Angiogenin (ANG), a 14-kDa basic protein is an angiogenic ribonuclease and member of the bovine pancreatic ribonuclease (RNase A) family (also known as RNase 5). Like RNase A, ANG cleaves preferentially on the 3′ side of pyrimidines and follows a transphosphorylation/hydrolysis mechanism. In addition, the crystal structure of human ANG has revealed that it has an RNase A fold and the catalytic triad (residues H13, K40 and H114) is conserved. The enzymatic activity of ANG is several orders of magnitude lower than that of RNase A towards conventional RNase substrates, but essential for its angiogenic effect.

ANG residues H13, K40 and H114 (part of the P1 sub-site) correspond to the catalytic triad. In the crystal structure of H13R ANG PD variant, the substitution of H13 by Arg is very clear in the electron density map and the overall structure is largely the same as with native ANG. In the native structure, Nδ1 of H13 forms a hydrogen bond with the main-chain O of T44 and Nε2 makes a water-mediated interaction with the amide nitrogen atom of L115. In the variant, the Arg side chain stretches out into the active site pocket making a direct interaction with Q117 while retaining its interactions with residues T44 and L115. The interaction with Q117 (known to be the obstructive pyrimidine-binding site residue in ANG)642 seem to result with slight rearrangement of the C-terminal helix. In addition, in the variant, the Arg side chain is not optimally positioned to interact with the two other catalytically important residues K40 and H114. This provides a structural explanation for the dramatic loss of RNase activity observed in this variant.

> MQDNSRYTHFLTQRYDAKPQGRDDRYCESIMRRRGLTSPCKDINTFIHGNKRSIKAICENKNGNPHRENLRISKSSFQVTTCKLHGGSPWPPCQYRATAGFRNVVVACENGLPVHLDQSIFRRP> MSTAAKQNRSTSRVSKKKTAAPKEGAAKKSDKGHKYEYVELAKASLTSAQPQHFYAVVIDATFPYKTNQERYICSLKIVDPTLYLKQQKGAGDASDYATLV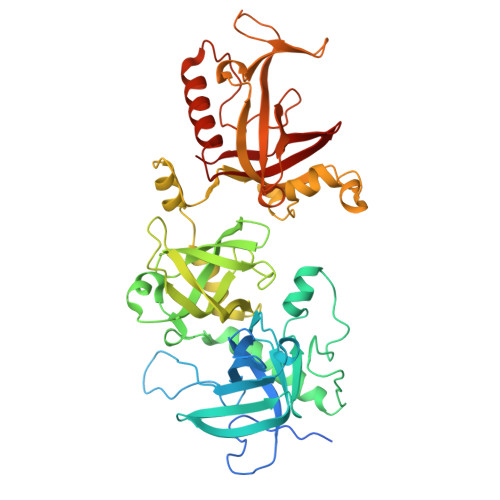LYAKRFEDLPIIHRAGDIIRVHRATLRLYNGQRQFNANVFYSSSWALFSTDKRSVTQEINNQDAVSDTTPFSFSSKHATIEKNEISILQNLRKWANQYFSSYSVISSDMYTALNKAQAQKGDFDVVAKILQVHELDEYTNELKLKDASGQVFYTLSLKLKFPHVRTGEVVRIRSATYDETSTQKKVLILSHYSNIITFIQSSKLAKELRAKIQDDHSVEVASLKKNVSLNAVVLTEVDKKHAALPSTSLQDLFHHADSDKELQAQDTFRTQFYVTKIEPSDVKEWVKGYDRKTKKSSSLKGASGKGDNIFQVQFLVKDASTQLNNNTYRVLLYTQDGLGANFFNVKADNLHKNADARKKLEDSAELLTKFNSYVDAVVERRNGFYLIKDTKLIY> QISDDFESGWDQTKWPISAPDCNQGGTVSLDTTVAHSGSNSMKVVGGPNGYCGHIFFGTTQVPTGDVYVRAWIRLQTALGSNHVTFIIMPDTAQGGKHLRIGGQSQVLDYNRESDDATLPDLSPNGIASTVTLPTGAFQCFEYHLGTDGTIETWL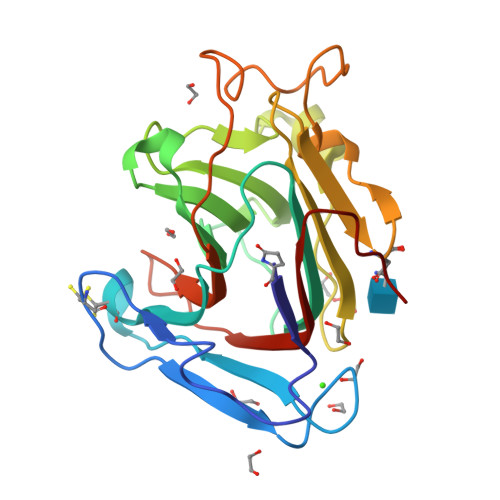NGSLIPGMTVGPGVDNPNDAGWTRASYIPEITGVNFGWEAYSGDVNTVWFDDISIASTRVGCG>[2x]MSLNNQDISIGKLSRLKIWITDNHLSDDQWSNTKKFIIIKITTEDGIEGWGEAFSINFREKGIAIIIKELFREISNIPNLSIKSFYNKISLLSDGHRGLDFSSATSAIEIALWDISGKLKNLPLNSLLTKSPKPNVPIYATCWSDLKKDTNDYLRQIEKFYGKKYGGIKIYPMLDSLS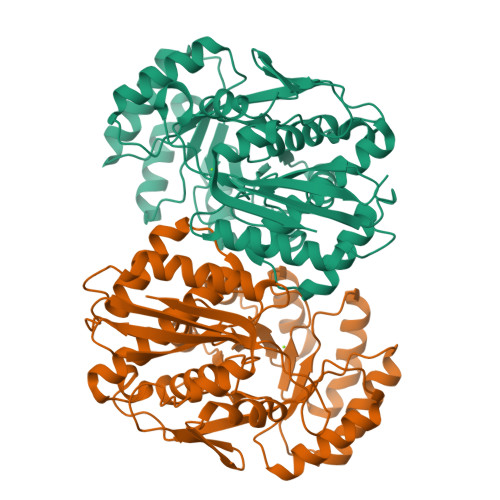ISIQFVEKVREIVGDELPLMLDLAVPEDLDQTKSFLKEVSSFNPYWIEEPVDGENISLLTEIKNTFNMKVVTGEKQSGLVHFRELISRNAADIFNPDISGMGGLIDIIEISNEASNNGIFISPHCWNSMSVSASAMLHVCSSIPNSEKAEIFPDYINFSKKFCELPFDIIDNKAHINKSAGLGIVIHEDILSELSIYSLDEKSNDEGHHHHHH> GSDEKRLHFGNGHL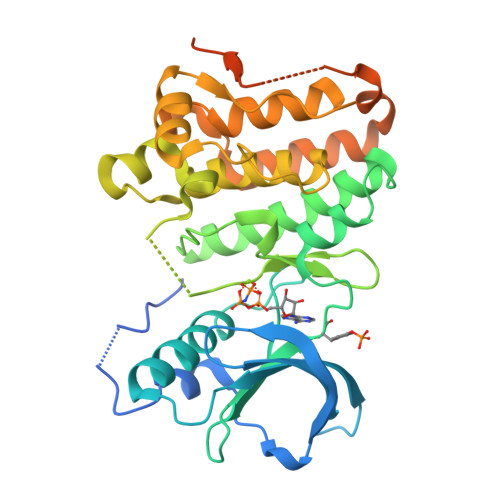KLPGLRTYVDPHTYEDPTQTVHEFAKELDATNISIDKVVGAGEFGEVCSGRLKLPSKKEISVAIKTLKVGYTEKQRRDFLGEASIMGQFDHPNIIRLEGVVTKSKPVMIVTEYMENGSLDSFLRKHDAQFTVIQLVGMLRGIASGMKYLSDMGYVHRDLAARNILINSNLVCKVSDFGLSRVLEDDPEAAYTTRGGKIPIRWTSPEAIAYRKFTSASDVWSYGIVLWEVMSYGERPYWEMSNQDVIKAVDEGYRLPPPMDCPAALYQLMLDCWQKDRNNRPKFEQIVSILDKLIRNPGSLKIITSAAARPSNLLLDQSNVDITTFRTTGDWLNGVWTAHCKEIFTGVEYSSCDTIAKIS> QDNSRYTHFLTQHYDAKPQGR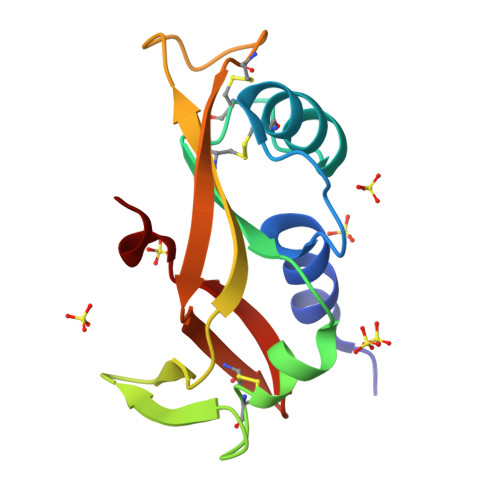DDRYCESIMRRRGLTSPCKDINTFIHGNKRSIKAICENKNGNPHRENLRISKSSFQVTTCKLHGGSPWPPCQYRATAGFRNVVVACENGLPVHLDQSIFR>GSHMASMKKKGSVVIVGRINLSGDTAYAQQTRGEEGCQETSQTGRDKNQVEGEVQIVSTATQTFLATSINGVLWTVYHGAGTRTIASPKGPVTQMYTNVDKDLVGWQAPQGSRSLTPCTCGSSDLYLVTRHADVIPVRRRGDSRGSLLSPRPISYLKGSAGGPLLCPAGHAVGIFKAAVSTRGVAKAVDFIPVESLETTMRSP[2x]

The HCV NS3/4A protease – a chymotrypsin-like serine protease – is a prime therapeutic target that cleaves four known sites along the virally encoded polyprotein. The NS3/4A protease also hydrolyzes two human proteins, TRIF and MAVS, which are part of the innate immune system, thereby confounding the innate immune response to viral infection. In this study, we report that four chemically representative protease inhibitors – telaprevir, danoprevir, vaniprevir and MK-5172 – exhibit distinct susceptibilities to the protease variants R155K, A156T and D168A. To elucidate the underlying mechanism by which chemically diverse inhibitors bind to the wild-type protease and drug-resistant variants, crystal structures were determined for 16 inhibitor-protease complexes. These complexes include wild-type protease and resistant variants R155K, D168A and A156T each bound to telaprevir, danoprevir, vaniprevir and MK-5172, with resolutions ranging from 1.10–2.50 Å; S139A protease variants were used except for telaprevir, which requires covalent bond formation with the serine 139 for efficient binding.

Vaniprevir, with the P2 isoindoline moiety, bound in a conformation similar to danoprevir, making favorable cation-π stacking interactions with R155, despite the P2–P4 macrocycle. Relative to the wild type, R155K caused large reductions in potency for danoprevir and vaniprevir, but MK-5172 remained highly active (R155K IC50 = 0.55 nM). For both danoprevir and vaniprevir, the R155K mutation disrupted the favorable cation-π stacking interactions with the P2 isoindoline moieties, causing significant reductions in drug potencies. R155K and D168A mutations confer danoprevir and vaniprevir resistance by disrupting favorable cation-π stacking interactions with R155. In danoprevir, the P2 isoindoline moiety shifted in response to R155K and D168A mutations, making extensive interactions with the catalytic D81. For vaniprevir, the rigidity of the P2–P4 macrocycle prevented similar compensatory changes. The flexible P2 isoindoline moiety of danoprevir containing a P1–P3 macrocycle packs against the mutated surfaces of A156T and D168A variants, explaining its relatively higher activity against both protease variants. However, the isoindoline moiety in vaniprevir is constrained due to the P2–P4 macrocycle, resulting in significantly lower activity against all three variants. The resistance at R155K occurs due to reduced interactions in the S2 subsite.>KVFERCELARTLKRLGMDGYRGISLANWMCLAKWESGYNTRATNYNAGDRSTDYGIFQIN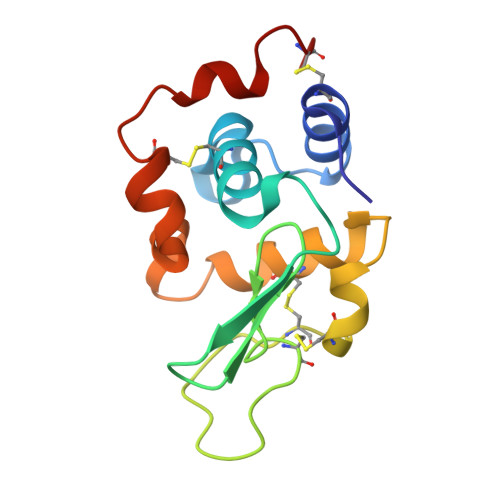SRYCANDGKTPGAVNACHLSCSALLQDNIADAVACAKRVVRDPQGIRAWVAWRNRCQNRDVRQYVQGCGV[4x]> QDRDWSSPQQPFTIYGNTHYVGTGGISAVLLSSPQGHILVDGTTEKGAQVVAANIRAMGFKLSDVKYILSTHSHEDHAGGISAMQKLTGATVLAGAANVDTLRTGVSPKSDP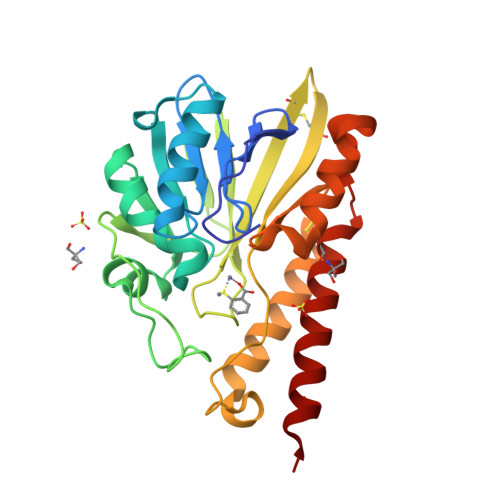QFGSLSNFPGSAKVRAVADGELVKLGPLAVKAHATPGHTEGGITWTWQSCEQGKCKDVVFADSLTAVSADSYRFSDHPEVVASLRGSFEAVEKLSCDIAIAAHPEVNDMWTRQQRAAKEGNSAYVDNGACRAIAAAGRKRLETRLASEKR> RLR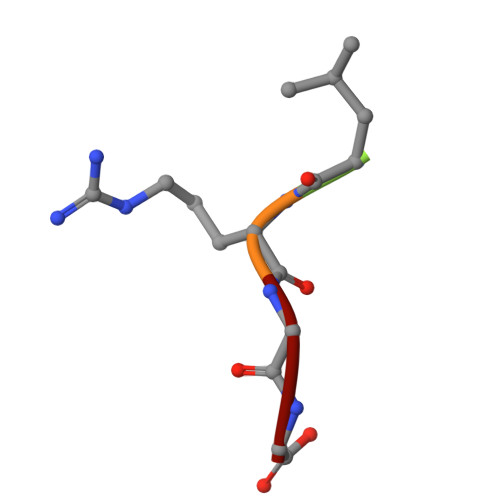GG>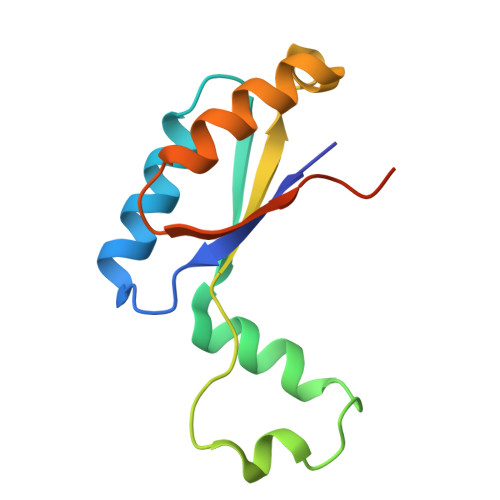 MGQITVYLQKTLDDDAAAGVVAQLQAEQGVEKVNYLSREDALGEFRNWSGFGGALDMLEENPLPAVAVVIPKLDFQGTESLNTLRDRITQINGIDEVRMDDSLEHHHHHH> ADLTASTTATATLVEPARITLTYKEGAPITIMDNGNIDTELLVGTLTLGGYKTGTTSTSVNFTDAAGDPMYLTFTSQDGNNHQFTTKVIGKDSRDFDISPKVNGE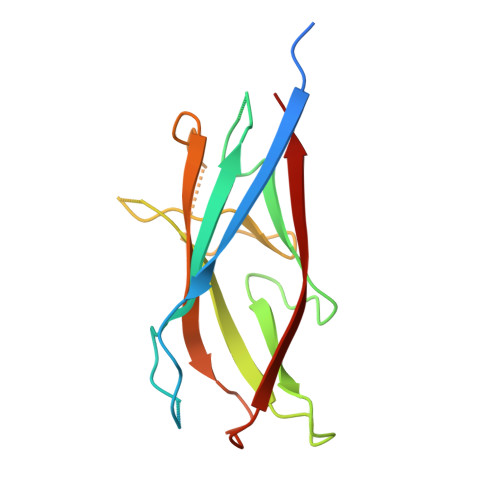NLVGDDVVLATGSQDFFVRSIGSKGGKLAAGKYTDAVTVTVSNQ>[2x]GTIGSMAAAPQVKTQAPGFYRMMLGDFEVTALSDGTVDLPVDKLLNQPPAKTQSALAKSFLKAPLETSVNAYLVNTGSKLVLVDTGAAGLFGPT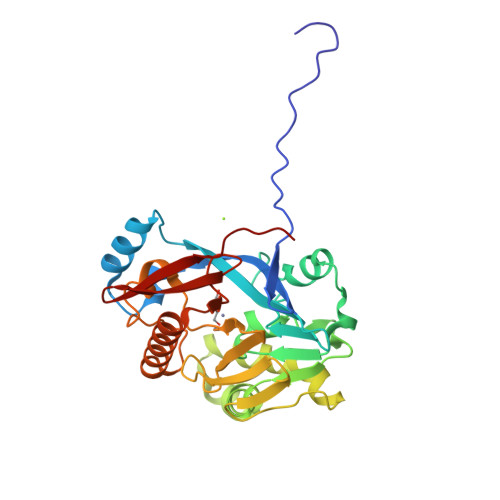LGKLAANLKAAGYQPEQVDEIYITHMHPDHVGGLMANEQAAFPNAVVRADQKDADFWLSQANLDKAPDDEKGFFQGAMASLNPYVKAGKFKPFSGNTDLVPGIKALASHGHTPGHTTYVVESKGQKLVLLGDLIHVAAVQFDDPSVTIQFDSDSKAAAAERKKAFADAAKGGYLIGAAHLSFPGIGHIRADGKGYRFVPVNYSVA>[2x]GSHMSDLPLRFPYGRPEFLGLSQDEVEASADHIARPILILKETRRLPWATGYAEVINAGKSTHNEDQASCEVLTVKKKAGAVTSTPNRNSSKRRSSLPNGEGLQLKENSESEGVSCHYWSLFDGHAGSGAAVVASRLLQHHITEQLQDIVDILKNSAVLGSGSTRFFTEKKIPHECLVIGALESAFKEMDLQIERERSSYNISGGCTALIVICLLGKLYVANAGDSRAIIIRNGEIIPMSSEFTPETERQRLQYLAFMQPHLLGNEFTHLEFPRRVQRKELGKKMLYRDFNMTGWAYKTIEDEDLKFPLIYGEGKKARVMATIGVTRGLGDHDLKVHDSNIYIKPFLSSAPEVRIYDLSKYDHGSDDVLILATDGLWDVLSNEEVAEAITQFLPNCDPDDPHRYTLAAQDLVMRARGVLKDRGWRISNDRLGSGDDISVYVIPLIHGNKLS

Recent work has shown that the metal‐dependent protein phosphatase PPM1H counteracts LRRK2 by dephosphorylating Rabs. The crystal structure of PPM1H reveals a structurally conserved phosphatase fold that strikingly has evolved a 110‐residue flap domain adjacent to the active site. Cellular assays, crosslinking and 3‐D modelling suggest that the flap domain encodes the docking motif for phosphorylated Rabs. Therefore, PPM1H has acquired a Rab‐specific interaction domain within a conserved phosphatase fold.

To grow WT crystals and improve diffraction, a “loop deletion” variant of PPM1H (PPM1H‐LD) was designed to eliminate a flexible and non‐conserved loop (188‐226) that was predicted to be distant from the active site. WT and D288A variants of PPM1H (PPM1HWT‐LD, PPM1HDA‐LD) diffracted to 2.5 Å and 2.6 Å resolution, respectively. The 2.5 Å model of PPM1HWT‐LD will be used for ensuing discussions, except for 3‐D docking analyses with model substrates in which we used the MnPPM1HWT‐LD variant. The structure of PPM1H adopts a conserved PPM fold consisting of 10 β‐strands organized into a 5 × 5 β‐sandwich. The active site cleft is formed by loops, including a short α‐helical loop (α4, residues 443–447), that connect β‐strands on one edge of the β‐sandwich. Three conserved aspartate residues—D151, D437 and D498—form direct contacts with two Mg2+ ions (M1 and M2) at the active site. M1 is coordinated by D437 and D498, while D151 coordinates both metal sites. The metal binding includes water molecules, and the geometry is approximately octahedral for both metal sites (M1 and M2). Deletion of the loop 188‐226 and the N‐terminus (1–32) does not affect the ability of PPM1HWT‐LD to dephosphorylate pRab8a relative to the full‐length enzyme in vitro and in cells (Fig EV1A and B). Using size exclusion chromatography coupled to multi‐angle light scattering (SEC‐MALS), we showed that PPM1HWT‐LD is a dimer.> RSPWCVICDPSVVLALKSLEKDYLP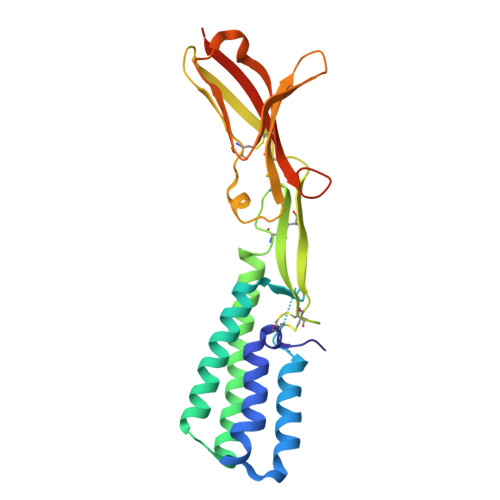GHLDAKHHKAMMERVENAVKDFQELSLNEDAYMGVVDEATLQKGSWSLLKDLKRITDSDVKGDLFVKELFWMLHLQKETFATYVARFQKEAYCPNKCGVMLQTLIWCKNCKKEVHACRKSYDCGERNVEVPQMEDMILDCELNWHQASEGLTDYSFYRVWGNNTETLVSKGKEATLTKPMVGPEDAGSYRCELGSVNSSPATIINFHVTVLPKEFLEVLFQ> SDDRFLREKQAKLAEKIREFNDARQRGTPFYICRDLADLESKSGDRHGPHIVEAYRAVMEMVGEHPDAGEAPRERQFAKMYLDPNTQSANALAMRKQILKGATTFLEKQFWNEVNSLIAKYPQDANLGGLPDVVSKIKAYIRLRIARKTLVPDNVELQQINGEYVWAIVFYLLRAGFVTEAAQYVNSNQAHFRAIDRTFSGYINSYASSEERRLKRQMQDRCMSEYNQRIRNAPEGSIDPFRMACYKIIGRCDLSNRSLDGLQTDVNDWIWLQFNLARETDRSLELAGESYGLAELQASIREIGLKHFPKTAAEDTNGSFGMFFYLQILAGMFEQAIAYLYPFSYVDAVHFAIALTYYGLLRPVDAASAGNELLSHNTRSMPQI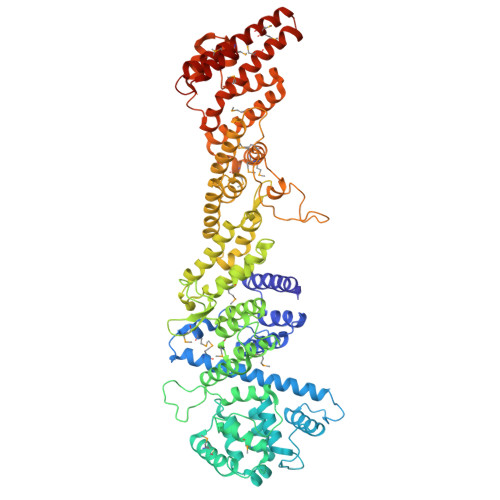NFGRMLGYYTRDFRAANPAAAVDYLVLICLNADEAAGGQQAQAALCHEALRELVLESREFSRLIGDIRPDGRRIRGVIEERGPLIALGQEDDFIRTITLQAASFADDNGRTTDAVLLYHLAEDYDTVVSIVSRALSEAISLEIGEDPMRLIPVKPRVTNAEGQVEEAAPGSSLSLAAIDDPVELAKAMMGMYERDHMFWQKIREPNRVACSVLLQMADIKSLVEQGRWAECLDKIRALDILPLTARGDPGTIRSYAARFPSLAQPVAINVPNLLMWTVLCCMRQRERLAGGQFAGNESTARLMMDELKQMTVDLMAYTSQLRYRLPPHLHEALARASAD>MSWQSYVDDHLMCEVEGNHLTHAAIFGQDGSVWAQSSAFPQLKPAEIAGINKDFEEAGHLAPTGLFLGGEKYMVVQG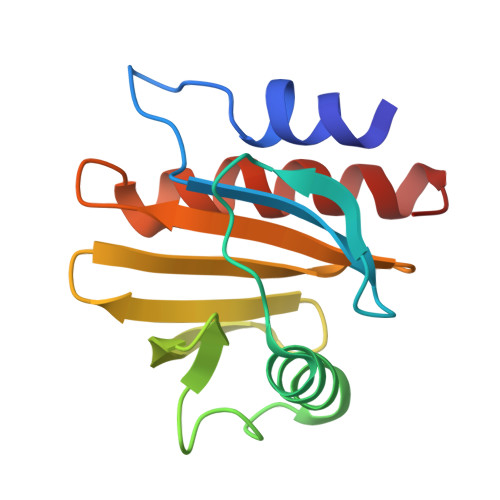EAGAVIRGKKGPGGVTIKKTTQALVFGIYDEPMTGGQCNLVVERLGDYLIESGL[2x]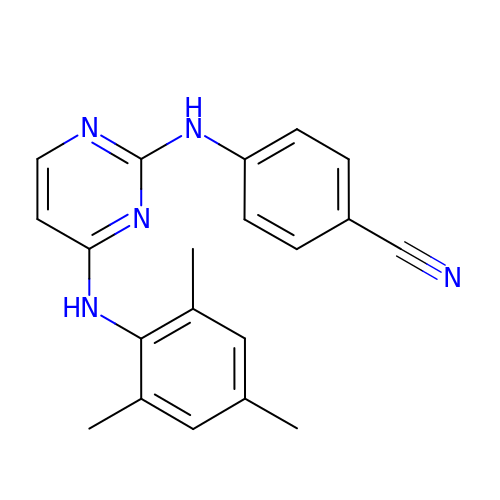4-[4-(2,4,6-TRIMETHYL-PHENYLAMINO)-PYRIMIDIN-2-YLAMINO]-BENZONITRILE | C20 H19 N5 | ILAYIAGXTHKHNT-UHFFFAOYSA-N> MHRVMGIETEYGISVPHQPNANAMAASSQVVNAYAPIGAPAQRQARWDFEEENPLRDARGFEVAREAADPSQLTDEDLGLANVILTNGARLYVDHAHPEYSTPEVTNPRDAVLWDKAGERIMAEAARRAADLPMGWTIQLYKNNTDNKGASYGCHENYLMNRSTPFADIVRHLIPFFVTRQVFCGAGRVGIGADGRGEGFQLS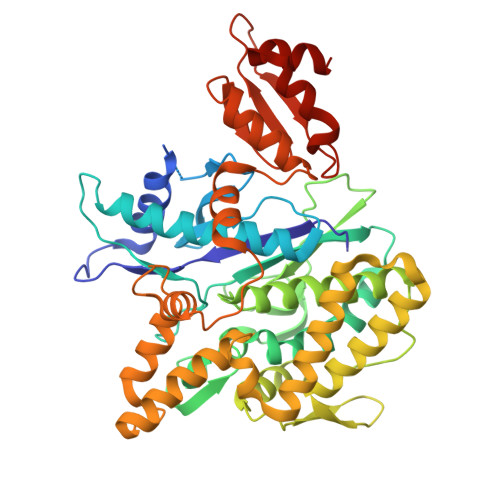QRADFFEVEVGLETTLKRPIINTRDEPHADPEKYRRLHVIIGDANMSEIATYLKLGTTALVLAMIEDGFLSQDFSVESPVGALRAVSHDPTLRYQLRLHDGRRLTAVQLQMEYLEQARKYVEDRFGTDVDDMTRDVLDRWETTLVRLADDPMQLSRDLDWVAKLSILEGYRQRENLPWSAHKLQLVDLQYHDVRPDRGLYNRLVARGRMNLLVDEAAVRTAMHEPPNDTRAYFRGRCLAKFGAEIAAASWDSVIFDLPGRDSLQRVPTLEPLRGTRAHVGDLLDRCRSATELVAALTGHHHHH> ADPLKSPQKVEVDIIDDNFILRWNRSDESVGNVTFSFDYQ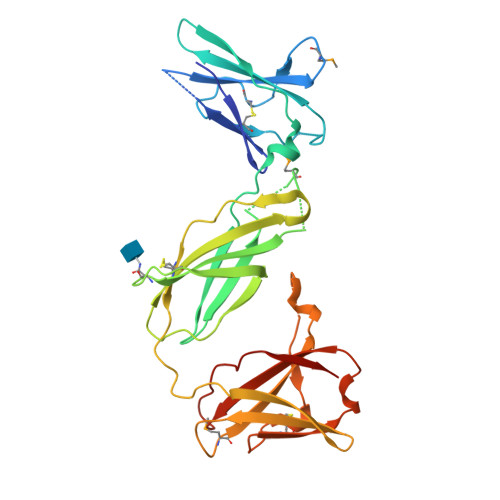KTGMDNWIKLSGCQNITSTKCNFSSLKLNVYEEIKLRIRAEKENTSSWYEVDSFTPFRKAQIGPPEVHLEAEDKAIVIHISPGTKDSVMWALDGLSFTYSLVIWKNSSGVEERIENIYSRHKIYKLSPETTYCLKVKAALLTSWKIGVYSPVHCIKTTVENELPPPENIEVSVQNQNYVLKWDYTYANMTFQVQWLHAFLKRNPGNHLYKWKQIPDCENVKTTQCVFPQNVFQKGIYLLRVQASDGNNTSFWSEEIKFDTEIQAFL5'-({[(2R,3R)-3-amino-2-{[2-({N-[(2R)-2-hydroxy-3,3-dimethyl-4-{[oxido(oxo)phosphonio]oxy}butanoyl]-beta-alanyl}amino)ethyl]sulfanyl}-4-methylpentyl]sulfonyl}amino)-5'-deoxyadenosine 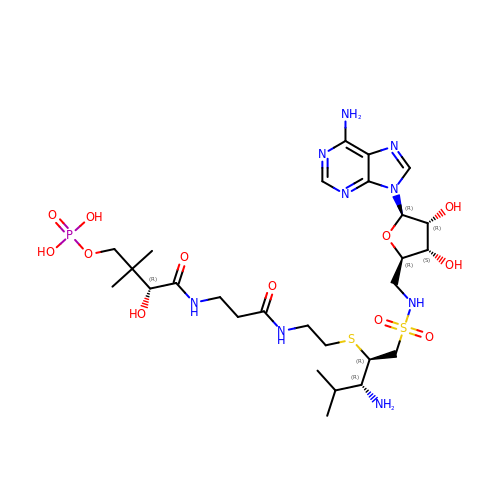| C27 H48 N9 O12 P S2 | LAWRAYXGFUHBCH-AWSFPXBRSA-N> MKKQYLKSGSGTRKEKDKAKRWFLDNGSIFLRELVADCNGKSIPIRSFSPEQILKATNNFDSSCFVSQDVYYKWYRGEIEDRSYMIKRFSEDEITGKRHRVKEVYNDIVLSARMSNHSNFLQLLGCCLEFPFPVLVFEFAEHGAMNQRGGVIVNGEESLLPWSVRLKIGKEIANAVTYLHTAFPKIIIHRDVKPMHVFLDKNWTAKLSDLSFSISLPEGKSRIEAEWVLGTFGYIDPLYHKTCFVTEYTDVYSFGICLLVIITGKPAIMTISDGDLQGILSLVRELCENG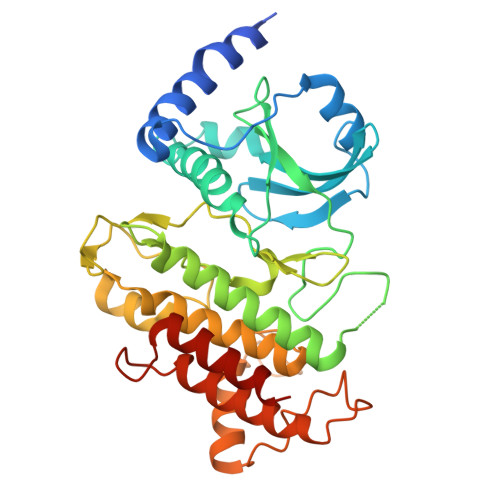KLDEVIDPRLMKDITSGQRLQVEACVVLALRCCKERDEDRPKMIQVAKELKQIEASLKNSS>MDKFRVQGPTRLQGEVTISGAKNAALPILFAALLAEEPVEIQNVPKLKDIDTTMKLLTQLGTKVERNGSVWIDASNVNNFSAPYDLVKTMRASIWALGPLVARFGQGQVSLPGGCAIGARPVDLHIFGLEKLGAEIKLEEGYVKASVNGRLKGAHIVMDKVSVGATVTIMSAATLAEGTTIIENAAREPEIVDTANFLVALGAKISGQGTDRITIEGVERLGGGVYRVLPDRIETGTFLVAAAISGGKIVCRNAQPDTLDAVLAKLREAG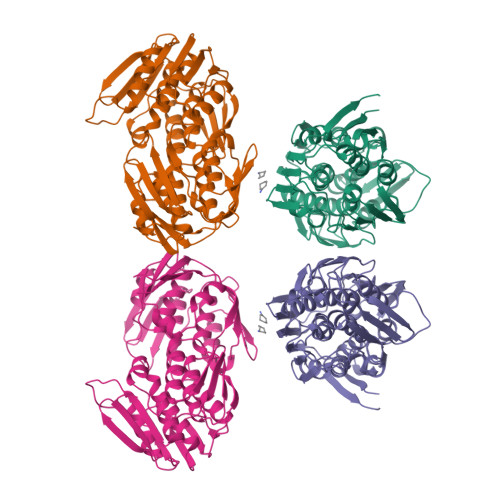ADIETGEDWISLDMHGKRPKAVTVRTAPHPAFPTDMQAQFTLLNLVAEGTGVITETIFENRFMHVPELIRMGAHAEIESNTVICHGVEKLSGAQVMATDLRASASLVLAGCIAEGTTVVDRIYHIDRGYERIEDKLRALGANIERVKGE[2x]> FHVKSGLQIKKNAIIDDYKVTSQVLGLGINGKVLQIFNKRTQEKFALKMLQDCPKARREVELHWRASQCPHIVRIVDVYENLYAGRKCLLIVMECLDGGELFSRIQDRGDQAFTEREASEIMKSIGEAIQYLHSINIAHRDVKPENLLYTSKRPNAILKLTDFGFAKETTSHNSLTTPCYTPYYVAPEVLGPEKY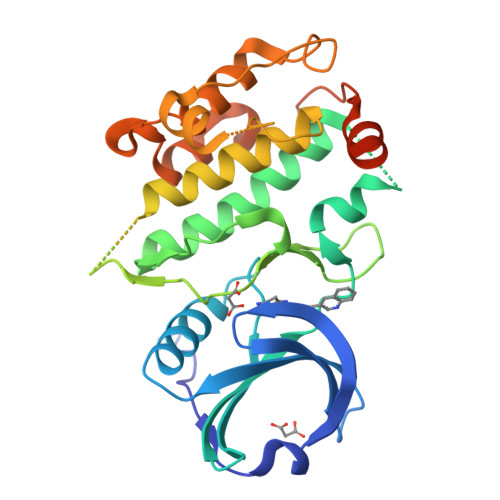DKSCDMWSLGVIMYILLCGYPPFYSNHGLAISPGMKTRIRMGQYEFPNPEWSEVSEEVKMLIRNLLKTEPTQRMTITEFMNHPWIMQSTKVPQTPLHTSRVLKEDKERWEDVKEEMTSALATMR2,6-bis[(4,6-dimethoxypyrimidin-2-yl)oxy]benzoic 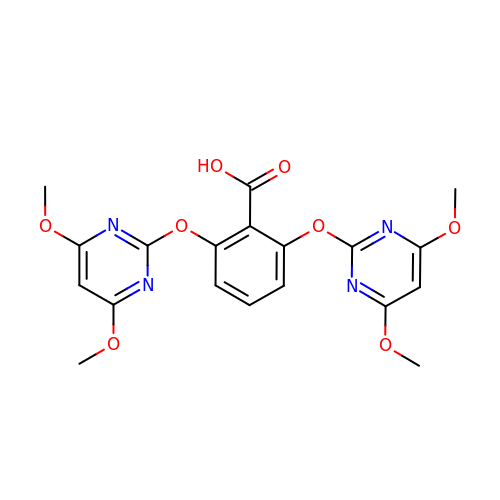acid | C19 H18 N4 O8 | RYVIXQCRCQLFCM-UHFFFAOYSA-N> MGNCNKPPKRPPNTQTSSNQPSAEFRRTAP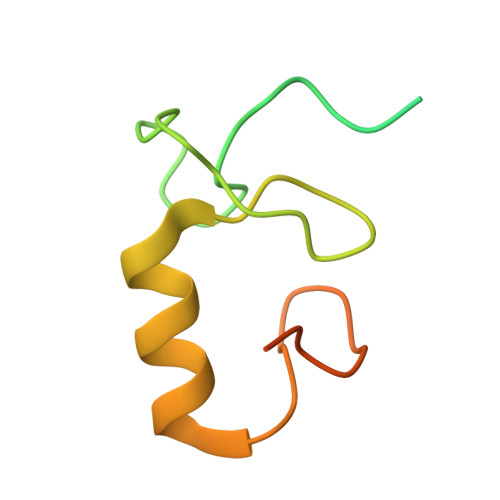PSLYGRYNCKCCWFADTNLITCNDHYLCLRCHQTMLRNSELCHICWKPLPTSITVPVEPSAPPP(2R,4S,6R)-4-amino-6-methyl-5-oxotetrahydro-2H-pyran-2-yl [(2R,3S,5R)-3-hydroxy-5-(5-methyl-2,4-dioxo-3,4-dihydropyrimidin-1(2H)-yl)tetrahydrofuran-2-yl]methyl dihydrogen diphosphate | C16 H25 N3 O13 P2 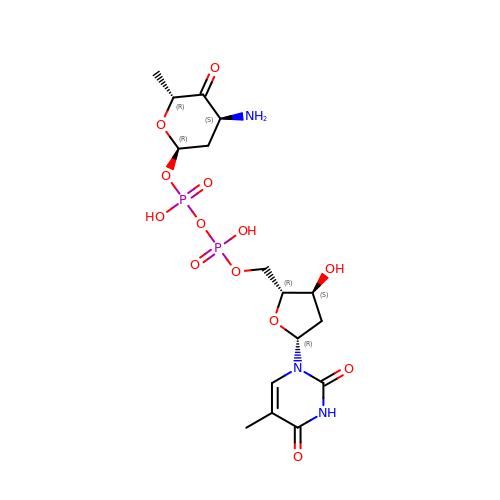| IVWGOICUSBJICO-KISRQWFGSA-N Notum is a carboxylesterase that suppresses Wnt signaling through deacylation of an essential palmitoleate group on Wnt proteins. Notum is a negative regulator of the Wnt signaling pathway. It is a secreted protein that functions as a carboxylesterase, removing a palmitoleate ester from a conserved serine residue in Wnt proteins that is essential for its binding and activation of the cell surface coreceptors. The structure of Notum has a clearly defined lipophilic pocket adjacent to the catalytic triad that accommodates a C16-lipid palmitoleate group of Wnt.

Exploration of the substituents on the aryl ring that binds in the palmitoleate pocket of Notum gave potent early lead 7y (IC50 9.5 nM) and further optimization of the triazole group delivered 8l (IC50 6.7 nM). So far, all changes to the C4 substituent had been unfavorable, then, somewhat unexpected, potent inhibition of Notum activity was entirely recovered by removal of the substituent as unsubstituted triazole 8l (IC50 6.7 nM) was the most potent inhibitor prepared in this series. The Notum-8l X-ray structure is consistent with the ligand retaining the H-bond between N3 of the triazole and the backbone of Trp128. In addition, 8l has near complete occupancy of the palmitoleate pocket through the 2-Cl-3-CF3-4-Cl substituents on the aryl ring. The near optimal filling of the pocket is achieved while still positioning the triazole in a favorable position for a hydrogen bond with the backbone of Trp128. This combination of features is likely why such high potency is observed. Triazole 8l restored Wnt signaling in the presence of Notum (EC50 110 nM) in a cell-based TCF/LEF reporter assay confirming functional activity. Assessment in broader off-target and safety pharmacology screens showed 8l to be selective against serine hydrolases, kinases, and representative drug targets. In summary, triazole 8l (ARUK3001185) is a potent and selective inhibitor of Notum activity with good brain penetration suitable for oral dosing in rodent models of disease.

> ETGSAQQLNEDLRLHLLLNTSVTCNDGSPAGYYLKESRGSRRWLLFLEGGWYCFNRENCDSRYDTMRRLMSSRDWPRTRTGTGILSSQPEENPYWWNANMVFIPYCSSDVWSGASSKSEKNEYAFMGALIIQEVVRELLGRGLSGAKVLLLAGSSAGGTGVLLNVDRVAEQLEKLGYPAIQVRGLADSGWFLDNKQYRHTDCVDTITCAPTEAIRRGIRYWNGVVPERCRRQFQEGEEWNCFFGYKVYPTLRSPVFVVQWLFDEAQLTVDNVHLTGQPVQEGLRLYIQNLGRELRHTLKDVPASFAPACLSHEIIIRSHWTDVQVKGTSLPRALHCWDRSLHDSHKASKTPLKGCPVHLVDSCPWPHCNPSCPTGTKHHHHHH>[6x]GSTAPPTNQWYHGKLDRTIAEERLRQAGKSGSYLIRESDRRPGSFV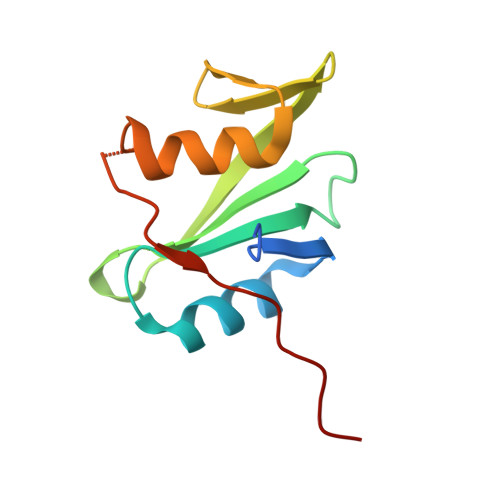LSFLSQMNVVNHFRIIAMSGDYYIGGRRFSSLSDLIGYYSHVSSLLKGEKLLYPVAPPEPVED The majority of traits controlled by rhl transcription factor RhlR depend on PqsE, a dispensable thioesterase in Pseudomonas Quinolone Signal (PQS) biosynthesis that interferes with RhlR through an enigmatic mechanism likely involving direct interaction of both proteins. Here we show that PqsE and RhlR form a 2:2 protein complex that, together with RhlR agonist N-butanoyl-L-homoserine lactone (C4-HSL), solubilizes RhlR and thereby renders the otherwise insoluble transcription factor active. PqsE is a thioesterase that triggers transcription of the RhlR regulon through a hitherto cryptic mechanism, which we identify here as involving a significant chaperone-like component that enhances the stability of RhlR via protein complex formation. In common with many other gram-negative bacteria, two QS circuits use N-acyl-L-homoserine lactones (HSLs) as autoinducers, namely N-(3-oxododecanoyl)-L-HSL (3-oxo-C12-HSL) and N-butanoyl-L-HSL (C4-HSL), which are produced by autoinducer synthases LasI and RhlI and activate the LuxR-type transcription factors LasR and RhlR, respectively.

Loss of interaction was also found for variant RhlR-P61, in which we back-mutated residues in the DNA-binding domain to the wildtype sequence to assess the RhlR-regulatory activity of the stabilized protein. We then used a RhlR-P61-encoding plasmid vector to transform a ΔpqsE/ΔrhlR/ΔrhlI triple mutant of P. aeruginosa PA14. Here, the production of pyocyanin was restored to wildtype levels and not significantly altered by C4-HSL or mBTL, demonstrating that the stabilized RhlR indeed acts independently of PqsE and of these ligands. Crystallization of RhlR-P61 with mBTL showed the ligand in a similar position and conformation as in the other crystal structures determined here.

>[2x]MRNDGGFLDWWEDLRSEMQSITDSQEVFAVLEKEVRRLGFDYYAYCVRHPIPFTRPRIFMFGNYPPAWQEHYQAQNYFAIDPTIRHCLRSGNHIVWSDDLFADAQELWDDARDYGLRHGATHSCMAPNGVMGFLSVARSSPAISPHEREELRLRMRCLIELLHQTLTELNHPSLQSNPVCLSHREREILQWTADGKSSGEIAIILSISESTVNFHHKNIQKKFDAPNKTLAAAYAAALGLI> MMKVTPIALLLAGVLASPLCAAGLDAQLTLVDGSTDDVRVNLTLTNTGDKPIRLLKWQLPGSDDAPLFLVERDGQPVSYEGALIKRAAPTDKDFQLLKAGQSLTVQAEVSGLYDMSAQGQYSIRYQLPARRKRPRAKQAQASESNAITLWVEGVNDERVQAKVAAAEPQAVAGSVSFSGRCTNTQKSDLLTALDAASGISNNASSYLAVDKPDGQRYRSWFGAYSSARWDQAETNFSKIKDAIDNKPLTFDCSCKQSYFAYVYPDQPYKVYLCKSFWTAPVTGSDSRAGTIVHQLSHFNVVAGTDD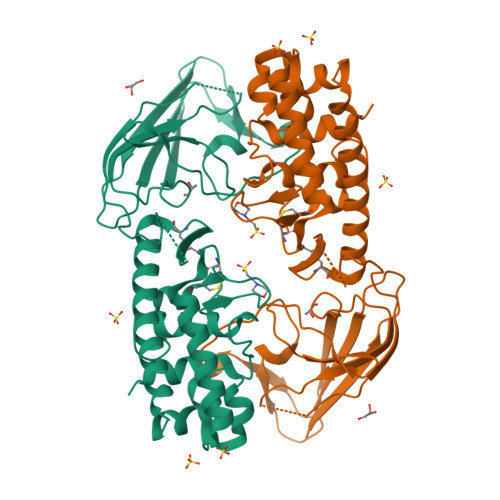LGYGQANARNLAKTDPVKALNNADNHEYFAENTPSEN(2R)-2,3-dihydroxypropyl 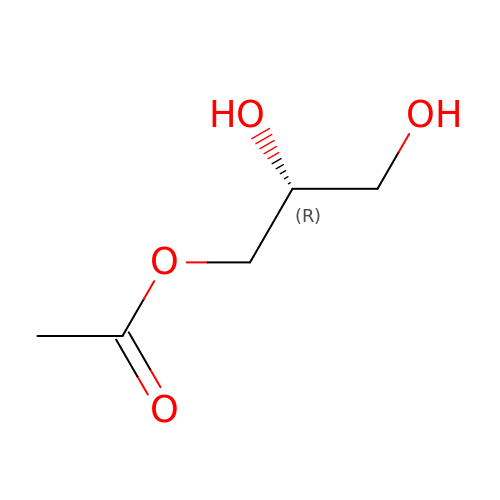acetate | C5 H10 O4 | KMZHZAAOEWVPSE-RXMQYKEDSA-N>GGCATGCC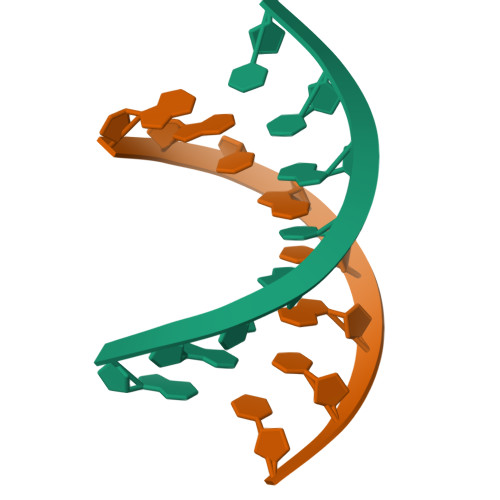[2x]>GPHMEMGRRIHLELRNRTPSDVKELVLDNSRSNEGKLEGLTDEFEELEFLSTINVGLTSIANLPKLNKLKKLELSDNRVSGGLEVLA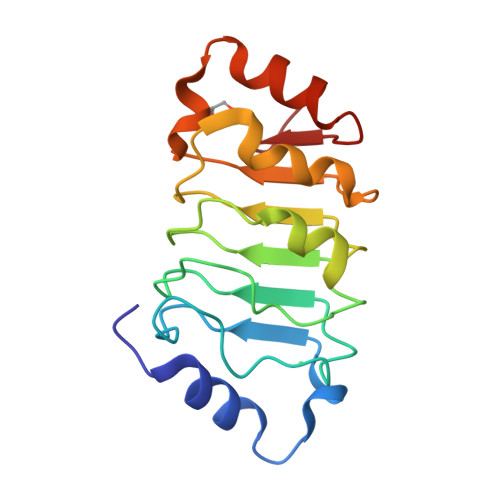EKCPNLTHLNLSGNKIKDLSTIEPLKKLENLKSLDLFNCEVTNLNDYRENVFKLLPQLTYLDGYD[2x]>MGSAFERVVRRVVQELDHGGEFIPVTSLQSSTGFQPYCLVVRKPSSSWFWKPRYKCVNLSIKDILEPDAAEPDVQRGRSFHFYDAMDGQIQGSVELAAPGQAKIAGGAAVSDSSSTSMNVYSLSVDPNTWQTLLHERHLRQPEHKVLQQLRSRGDNVYVVTEVLQTQKEVEVTRTHKREGSGRFSLPGATCEQGEGQGHLSQKKTVTIPSG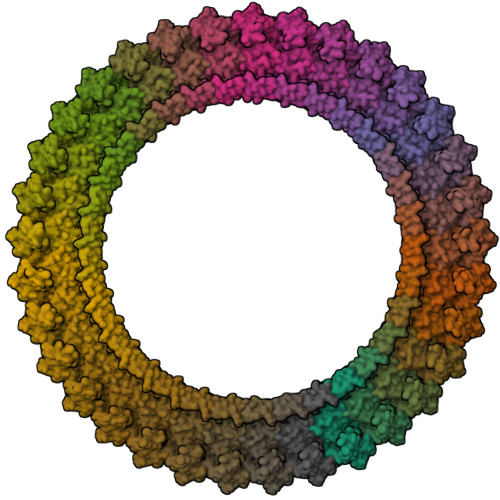STLAFRVAQLVIDSDLDVLLFPDKKQRTFQ[33x]>[2x]MPEGPSLRKFHQLVAPFVGQLVVTVGGNSKKINPNMLEMLRLQDSQVHGKNLYLNFGLTEDLGLPESFLLPKHLQKKVRLPKEKSDHKLETTSRLDGQEVPGSSLAIKALELGEEEKETVMPWWLNTSQNSGLWLCFHFGLFGSVRASELSRATKANKRGDWKDPIPRLVLHFAKGFLAFYNCRIYWCLGPTVKPTSDILSEEFDRRQALEALKQASPVSYTLLDQRYFAGLGNIIKNEVL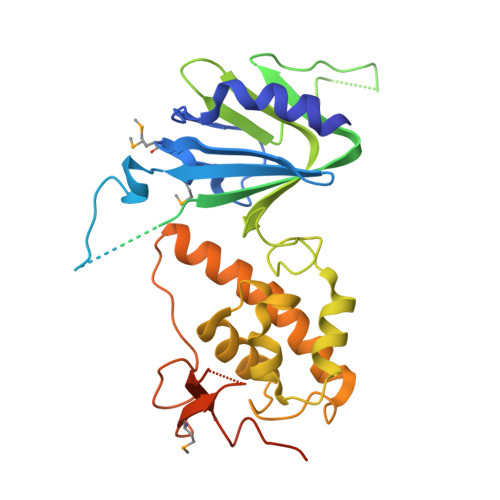YLARIHPLSLGSCLTPLNLESLLDHVVSFSVGWLQKKLEGKPLHHLIYQKEQCPAGHQVMKDSFGPPGSFQRLTWWCPHCQPKAEEKVEVTQEQLLEHHHHHH N-methyl-D-alaninamide | C4 H10 N2 O | 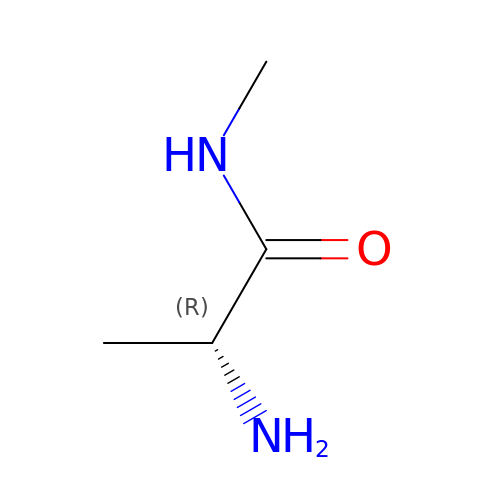CKQYFZPCICOPMQ-GSVOUGTGSA-N>MNSVVNNILKAHPHQTKSFYVSSPKIVEDLIDQWTILFPRVTPHYAVKCNNDEVLLKTMCDKNVNFDCASSSEIKKVIQIGVSPSRIIFAHTMKTIDDLIFAKDQGVDIATFDSSFELDKIHTYHPNCKMILRIRCDDPNATVQLGNKFGANEDEIRHLLEYAKQLDIEVIGISFHVGSGSRNPEAYYRAIKSSKEAFNEAISVGHKPYILDIGGGLHADI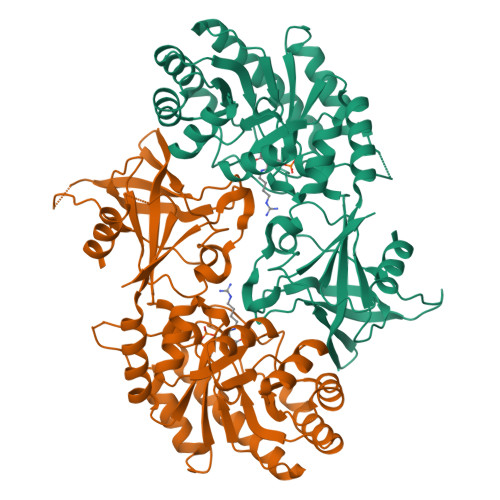DEGELSTYMSDYINDAIKDFFPEDTVTIVAEPGRFFAEHYSVLATQVIGKRVRDGLYEYFFNESTYGGFSNVIFEKSVPTPQLLRDVPDDEEYVPSVLYGCTCDGVDVINHNVALPELHIGDWVYFPSWGAYTNVLTTSFNGFGEYDVYYI[8x]>[2x]SNAMTS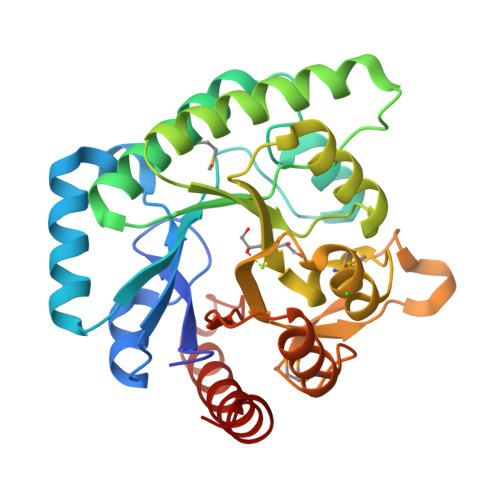HKPYWPIGVFTSVDAGLGVHLEVAQDLKVPTVQVHAPHPHTRTREHAQAFRAKCDAAGIQVTVIFGGFDGESYADIPTTARTVGLVPLETRASRVAEMKEISDFASWVGCPAIGLHIGFVPESSSPDYSELVRVTQDLLTHAANHGQAVHLETGQESADHLLEFIEDVNRPNLGINFDPANMILYGTGNPIEALRKVARYVRSIHCKDALWAPVNERGKSWGQEVALGTGDVGMEAYLTTLWEIGYRGPLTIEREIPHDPVQQKKDLASALELLTGLRKKIANC(3~{R})-4-ethyl-3-methyl-3-propyl-1~{H}-1,4-benzodiazepine-2,5-dione 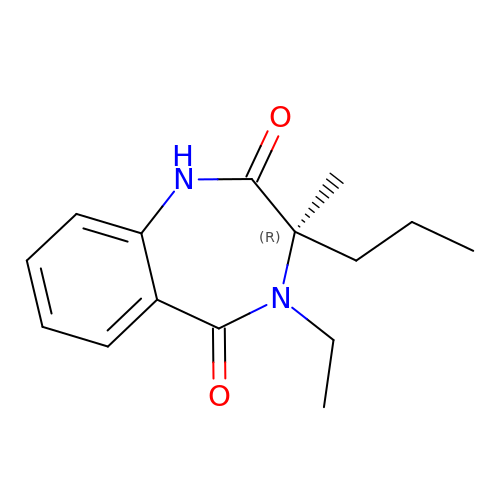| C15 H20 N2 O2 | QTYBGLRTPWRNRA-OAHLLOKOSA-N> MTTRNDCLALDAQDSLAPLRQQFALPEGVIYLDGNSLGARPVAALARAQAVIAEEWGNGLIRSWNSAGWRDLSERLGNRLATLIGARDGEVVVTDTTSINLFKVLSAALRVQATRSPERRVIVTETSNFPTDLYIAEGLADMLQQGYTLRLVDSPEELPQAIDQDTAVVMLTHVNYKTGYMHDMQALTALSHECGALAIW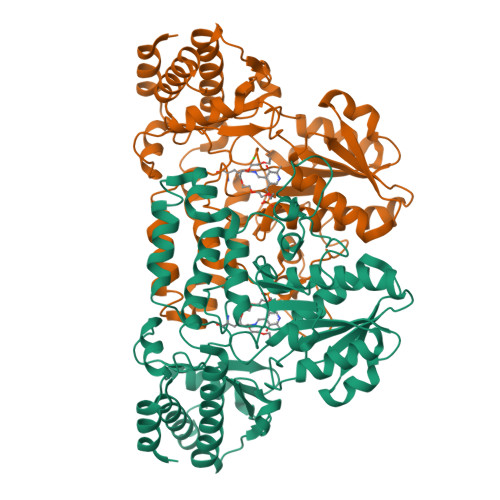DLAHSAGAVPVDLHQAGADYAIGCTYKYLNGGPGSQAFVWVSPQLCDLVPQPLSGWFGHSRQFAMEPRYEPSNGIARYLCGTQPITSLAMVECGLDVFAQTDMASLRRKSLALTDLFIELVEQRCAAHELTLVTPREHAKRGSHVSFEHPEGYAVIQALIDRGVIGDYREPRIMRFGFTPLYTTFTEVWDAVQILGEILDRKTWAQAQFQVRHSVT[[(2~{R},3~{S},4~{R},5~{R})-5-(6-aminopurin-9-yl)-3,4-bis(oxidanyl)oxolan-2-yl]methoxy-oxidanyl-phosphoryl] ethanoate | C12 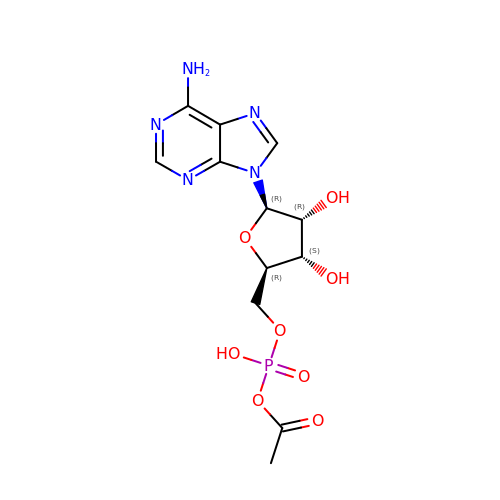H16 N5 O8 P | UBPVOHPZRZIJHM-WOUKDFQISA-N>[2x]MSKGEKMKIKVGVLGATGSVGQRFVQLLADHPMFELTALAASERSAGKKYKDACYWFQDRDIPENIKDMVVIPTDPKHEEFEDVDIVFSALPSDLAKKFEPEFAKEGKLIFSNASAYRMEEDVPL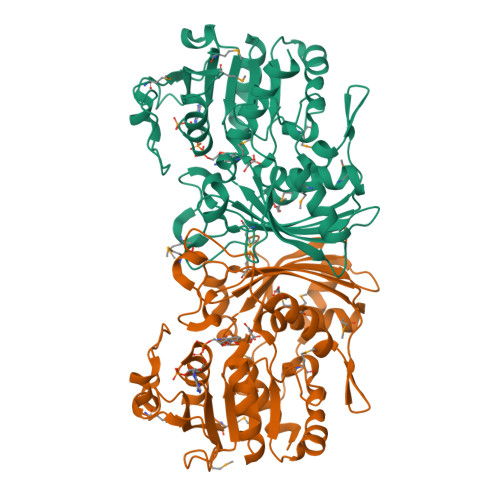VIPEVNADHLELIEIQREKRGWDGAIITNPNCSTICAVITLKPIMDKFGLEAVFIATMQAVSGAGYNGVPSMAILDNLIPFIKNEEEKMQTESLKLLGTLKDGKVELANFKISASCNRVAVIDGHTESIFVKTKEGAEPEEIKEVMDKFDPLKDLNLPTYAKPIVIREEIDRPQPRLDRNEGNGMSIVVGRIRKDPIFDVKYTALEHNTIRGAAGASVLNAEYFVKKYI5-[2-(cyclohexylamino)pyridin-4-yl]-4-naphthalen-2-yl-2-(tetrahydro-2H-pyran-4-yl)-2,4-dihydro-3H-1,2,4-triazol-3-one | C28 H31 N5 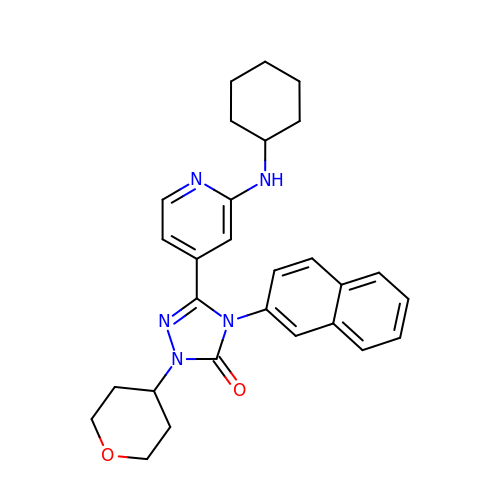O2 | YZJYYYWPZRYBLV-UHFFFAOYSA-N(2R,3S,4S,5R,6R)-6-dodecoxy-5-fluoranyl-2-(hydroxymethyl)oxane-3,4-diol | C18 H35 F O5 | 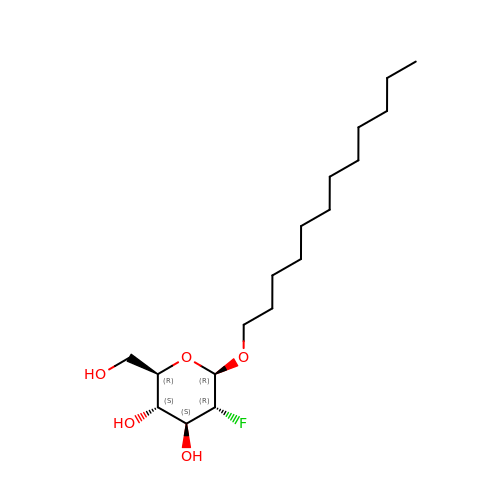WREKVDBUBSBPMM-DUQPFJRNSA-N9,9,9-TRIFLUORO-8-OXO-N-PHENYLNONANAMIDE 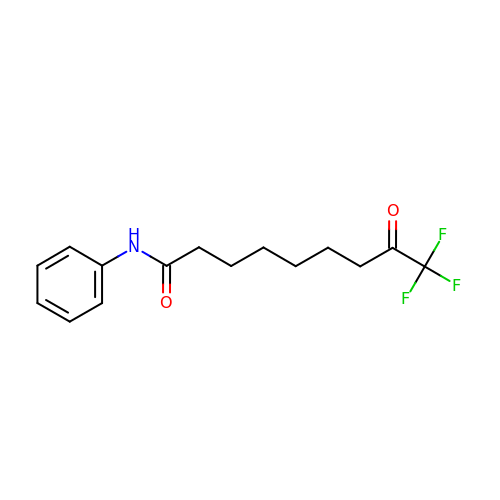| C15 H18 F3 N O2 | KRCXZGYVOZSCSF-UHFFFAOYSA-N>[2x]MSQRITIDPVTRIEGHLRIDCEIENGVVSKAWASGTMWRGMEEIVKNRDPRDAWMIVQRICGVCTTTHALSSVRAAESALNIDVPVNAQYIRNIILAAHTTHDHIV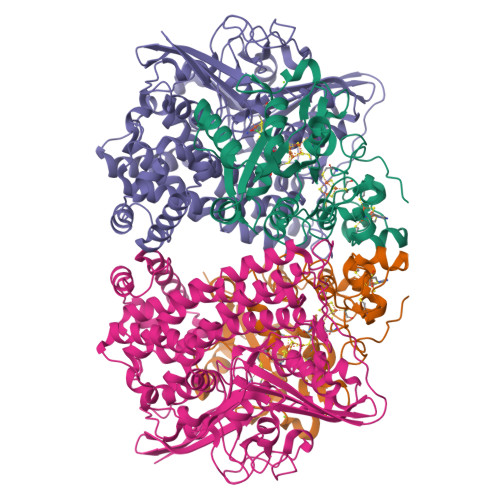HFYQLSALDWVDITSALQADPTKASEMLKGVSTWHLNSPEEFTKVQNKIKDLVASGQLGIFANGYWGHPAMKLPPEVNLIAVAHYLQALECQRDANRVVALLGGKTPHIQNLAVGGVANPINLDGLGVLNLERLMYIKSFIDKLSDFVEQVYKVDTAVIAAFYPEWLTRGKGAVNYLSVPEFPTDSKNGSFLFPGGYIENADLSSYRPITSHSDEYLIKGIQESAKHSWYKDEAPQAPWEGTTIPAYDGWSDDGKYSWVKSPTFYGKTVEVGPLANMLVKLAAGRESTQNKLNEIVAIYQKLTGNTLEVAQLHSTLGRIIGRTVHCCELQDILQNQYSALITNIGKGDHTTFVKPNIPATGEFKGVGFLEAPRGMLSHWMVIKDGIISNYQAVVPSTWNSGPRNFNDDVGPYEQSLVGTPVADPNKPLEVVRTIHSFDPCMACAVH;>[2x]MEMAESVTNPQRPPVIWIGAQECTGCTESLLRATHPTVENLVLETISLEYHEVLSAAFGHQVEENKHNALEKYKGQYVLVVDGSIPLKDNGIYCMVAGEPIVDHIRKAAEGAAAIIAIGSCSAWGGVAAAGVNPTGAVSLQEVLPGKTVINIPGCPPNPHNFLATVAHIITYGKPPKLDDKNRPTFAYGRLIHEHCERRPHFDAGRFAKEFGDEGHREGWCLYHLGCKGPETYGNCSTLQFCDVGGVWPVAIGHPCYGCNEEGIGFHKGIHQLANVENQTPRSQKPDVNAKEGGHHHHHH>[6x]GAMGNQKTKASKLETAAKNLENQNKQEYIKINEIDAQGINFLATFKADEKDNLSQYEEMQIKRTIYSSLNYEKQKINTLKEILETLYNKLQHRYTSKEFIYQIVASIQYDIDRVLCLIKEAIIKDNLHTQNQKESELLMNLDSSLKTRQNFAKKLNETIDDYNKDSKNIQTNVDALATYMKENYKTLDSFKPIN

Two CspA orthologous proteins, BGA71 and BGA66, that are capable of binding complement system components C7, C8, and C9 and thus inhibiting the assembly of the MAC have been identified in B. bavariensis, allowing B. bavariensis to escape the attack by the immune system. The importance of BGA71 and BGA66 in the resistance to the immune system was supported by the gain of resistance to complement-mediated killing after expression of either protein in the serum-sensitive B. garinii strain G132. In conclusion, we have solved the crystal structure of the key complement inhibitory protein BGA71 from B. bavariensis. The overall fold of the BGA71 protein looks similar (Cα root-mean-square deviation from 1.66 Ǻ to 2.63 Ǻ) to the previously released crystal structures of the orthologous PFam54 proteins CspA, BBA64, BBA66, and BBA73 of B. burgdorferi.

All three BGA71 constructs were overexpressed in E. coli, but only BGA7162-251 yielded crystals, suggesting that the flexible region present in the other two constructs interfered with the crystal formation, as previously observed for the BBA66 protein of B. burgdorferi. The crystals used for collection of native diffraction data also belonged to the space group P31, but the unit cell size was smaller and only six molecules were found per asymmetric unit with a water content of approximately 45%. The final model of BGA7162-251 was generated for residues 69–251 since the first four residues that remained after cleavage of the His-tag and residues 66–68 were not built due to weak electron density. By surveying the crystal structure of BGA71, we identified cysteine 173 in α-helix D as the residue that forms disulfide bridges, which is responsible for cross-linking of the two monomers. Furthermore, comparative sequence analysis of the PFam54 orthologous proteins reveals that cysteine 173 is not present in any other orthologous PFam54 protein, suggesting that dimerization by cysteine cross-linking is a unique feature of BGA71. The structure of CspA showed the highest similarity to BGA71 among the other PFam54 orthologs of B. burgdorferi, with a Cα root-mean-square deviation of 1.66 Ǻ. While BGA71 did not bind CFH and CFHL-1, an interaction with components C7 and C9 has been demonstrated. However, the lack of binding complement regulators can be explained by the inability of BGA71 to form a homodimer in the same manner as CspA. However, the proposed N-terminal residues 37–63 involved in the binding of C7 and C9 are not visible in the crystal structure of BGA71 since they form a flexible loop region connecting the protein structural domain to the cell surface.The S. cerevisiae respiratory SC is composed of complexes III2 (CIII, dimer of cytochrome bc1) and IV (CIV, Cyt c oxidase) with CIII flanked on each side by CIV in the core tetrameric SC (IV1III2IV1). CL is distinguished from other phospholipids by its unique dimeric structure containing two phosphates, four fatty acids and a free hydroxyl at the 2-position of the glycerol linking the two phosphatidyl groups. This unique dimeric structure makes CL ideal for supporting the organization of individual protein subunits into multi-subunit complexes, as well as individual complexes into supercomplex (SC) molecular machines, such as the mitochondrial respirasome. A presumed advantage in SC formation is bringing active sites of CIII and CIV in close proximity to each other to facilitate Cyt c shuttling of electrons. Here we show that anionic phospholipids interact with positive amino acids and appear to nucleate a phospholipid domain at the interface between the individual complexes, which dampen charge repulsion and further stabilize interaction, respectively, between individual complexes.

To address whether PG substitutes for CL in SC formation, we performed single-particle cryo-EM analysis of the trimeric SC purified from CRD1∆ cells. There was no density in the region of the CRD1∆ density map corresponding to the position of the Qcr10 subunit of CIII in the WT SC density map; we assume that this subunit was lost during purification. Densities for UQ6 were found only at Qi sites. The Qo sites were empty, which may be due to use of chromatography for purification resulting in the oxidation of UQ6. Analysis of the cryo-EM density for Rip1 subunit of CIII showed that both the hinge region and the head domain displayed weaker or less ordered density when compared to the WT. Our structural determination of the trimeric SC from CRD1∆ cells shows the presence of the anionic phospholipid PG at all CL positions found in the WT SC, which has been postulated but never demonstrated. PGT501J/j appears to replace the internal CLs in each monomer of CIII surprisingly resulting in little noticeable structural changes for CIII. PGT601K appears to only interact with CIV unlike CDL601K which interacts with both CIII and CIV. However, there is no interaction with Lys51 of Rip1 since PGT lacks a second phosphate. However, there were significant differences as to which amino acids interact with PG and none of the PGs formed interactions that bridge CIII and CIV.

>[2x]MLRTVTSKTVSNQFKRSLATAVATPKAEVTQLSNGIVVATEHNPSAHTASVGVVFGSGAANENPYNNGVSNLWKNIFLSKENSAVAAKEGLALSSNISRDFQSYIVSSLPGSTDKSLDFLNQSFIQQKANLLSSSNFEATKKSVLKQVQDFEENDHPNRVLEHLHSTAFQNTPLSLPTRGTLESLENLVVADLESFANNHFLNSNAVVVGTGNIKHEDLVNSIESKNLSLQTGTKPVLKKKAAFLGSEVRLRDDTLPKAWISLAVEGEPVNSPNYFVAKLAAQIFGSYNAFEPASRLQGIKLLDNIQEYQLCDNFNHFSLSYKDSGLWGFSTATRNVTMIDDLIHFTLKQWNRLTISVTDTEVERAKSLLKLQLGQLYESGNPVNDANLLGAEVLIKGSKLSLGEAFKKIDAITVKDVKAWAGKRLWDQDIAIAGTGQIEGLLDYMRIRSDMSMMRW;>[2x]MLSAARLQFAQGSVRRLTVSARDAPTKISTLAVKVHGGSRYATKDGVAHLLNRFNFQNTNTRSALKLVRESELLGGTFKSTLDREYITLKATFLKDDLPYYVNALADVLYKTAFKPHELTESVLPAARYDYAVAEQCPVKSAEDQLYAITFRKGLGNPLLYDGVERVSLQDIKDFADKVYTKENLEVSGENVVEADLKRFVDESLLSTLPAGKSLVSKSEPKFFLGEENRVRFIGDSVAAIGIPVNKASLAQYEVLANYLTSALSELSGLISSAKLDKFTDGGLFTLFVRDQDSAVVSSNIKKIVADLKKGKDLSPAINYTKLKNAVQNESVSSPIELNFDAVKDFKLGKFNYVAVGDVSNLPYLDEL;>MLGIRSSVKTCFKPMSLTSKRLISQSLLASKSTYRTPNFDDVLKENNDADKGRSYAYFMVGAMGLLSSAGAKSTVETFISSMTATADVLAMAKVEVNLAAIPLGKNVVVKWQGKPVFIRHRTPHEIQEANSVDMSALKDPQTDADRVKDPQWLIMLGICTHLGCVPIGEAGDFGGWFCPCHGSHYDISGRIRKGPAPLNLEIPAYEFDGDKVIVG[2x];>MSFSSLYKTFFKRNAVFVGTIFAGAFVFQTVFDTAITSWYENHNKGKLWKDVKARIAAGDGDDDDE[2x];>MPQSFTSIARIGDYILKSPVLSKLCVPVANQFINLAGYKKLGLKFDDLIAEENPIMQTALRRLPEDESYARAYRIIRAHQTELTHHLLPRNEWIKAQEDVPYLLPYILEAEAAAKEKDELDNIEVSK[2x];>[2x]MGMLELVGEYWEQLKITVVPVVAAAEDDDNEQHEEKAAEGEEKEEENGDEDEDEDEDEDDDDDDDEDEEEEEEVTDQLEDLREHFKNTEEGKALVHHYEECAERVKIQQQQPGYADLEHKEDCVEEFFHLQHYLDTATAPRLFDKLK;>MGPPSGKTYMGWWGHMGGPKQKGITSYAVSPYAQKPLQGIFHNAVFNSFRRFKSQFLYVLIPAGIYWYWWKNGNEYNEFLYSKAGREELERVNV[2x];>[2x]MAFRKSNVYLSLVNSYIIDSPQPSSINYWWNMGSLLGLCLVIQIVTGIFMAMHYSSNIELAFSSVEHIMRDVHNGYILRYLHANGASFFFMVMFMHMAKGLYYGSYRSPRVTLWNVGVIIFILTIATAFLGYCCVYGQMSHWGATVITNLFSAIPFVGNDIVSWLWGGFSVSNPTIQRFFALHYLVPFIIAAMVIMHLMALHIHGSSNPLGITGNLDRIPMHSYFIFKDLVTVFLFMLILALFVFYSPNTLGHPDNYIPGNPLVTPASIVPEWYLLPFYAILRSIPDKLLGVITMFAAILVLLVLPFTDRSVVRGNTFKVLSKFFFFIFVFNFVLLGQIGACHVEVPYVLMGQIATFIYFAYFLIIVPVISTIENVLFYIGRVNK;> MVQRWLYSTNAKDIAVLYFMLAIFSGMAGTAMSLIIRLELAAPGSQYLHGNSQLFNVLVVGHAVLMIFFLVMPALIGGFGNYLLPLMIGATDTAFPRINNIAFWVLPMGLVCLVTSTLVESGAGTGWTVYPPLSSIQAHSGPSVDLAIFALHLTSISSLLGAINFIVTTLNMRTNGMTMHKLPLFVWSIFITAFLLLLSLPVLSAGITMLLLDRNFNTSFFEVSGGGDPILYEHLFWFFGHPEVYILIIPGFGIISHVVSTYSKKPVFGEISMVYAMASIGLLGFLVWSHHMYIVGLDADTRAYFTSATMIIAIPTGIKIFSWLATIHGGSIRLATPMLYAIAFLFLFTMGGLTGVALANASLDVAFHDTYYVVGHFHYVLSMGAIFSLFAGYYYWSPQILGLNYNEKLAQIQFWLIFIGANVIFFPMHFLGINGMPRRIPDYPDAFAGWNYVASIGSFIATLSLFLFIYILYDQLVNGLNNKVNNKSVIYNKAPDFVESNTIFNLNTVKSSSIEFLLTSPPAVHSFNTPAVQS;>[2x]MFSNLSKRWAQRTLSKSFYSTATGAASKSGKLTQKLVTAGVAAAGITASTLLYADSLTAEAMTAAEHGLHAPAYAWSHNGPFETFDHASIRRGYQVYREVCAACHSLDRVAWRTLVGVSHTNEEVRNMAEEFEYDDEPDEQGNPKKRPGKLSDYIPGPYPNEQAARAANQGALPPDLSLIVKARHGGCDYIFSLLTGYPDEPPAGVALPPGSNYNPYFPGGSIAMARVLFDDMVEYEDGTPATTSQMAKDVTTFLNWCAEPEHDERKRLGLKTVIILSSLYLLSIWVKKFKWAGIKTRKFVFNPPKPRK;> MLCQQMIRTTAKRSSNIMTRPIIMKRSVHFKDGVYENIPFKVKGRKTPYALSHFGFFAIGFAVPFVACYVQLKKSGAF;> MANKVIQLQKIFQSSTKPLWWRHPRSALYLYPFYAIFAVAVVTPLLYIPNAIRGIKAKKA;> MTHLERSRHQQHPFHMVMPSPWPIVVSFALLSLALSTALTMHGYIGNMNMVYLALFVLLTSSILWFRDIVAEATYLGDHTMAVRKGINLGFLMFVLSEVLIFAGLFWAYFHSAMSPDVTLGACWPPVGIEAVQPTELPLLNTIILLSSGATVTYSHHALIAGNRNKALSGLLITFWLIVIFVTCQYIEYTNAAFTISDGVYGSVFYAGTGLHFLHMVMLAAMLGVNYWRMRNYHLTAGHHVGYETTIIYTHVLDVIWLFLYVVFYWWGV;> MLDLLRLQLTTFIMNDVPTPYACYFQDSATPNQEGILELHDNIMFYLLVILGLVSWMLYTIVMTYSKNPIAYKYIKHGQTIEVIWTIFPAVILLIIAFPSFILLYLCDEVISPAMTIKAIGYQWYWKYEYSDFINDSGETVEFESYVIPDELLEEGQLRLLDTDTSMVVPVDTHIRFVVTAADVIHDFAIPSLGIKVDATPGRLNQVSALIQREGVFYGACSELCGTGHANMPIKIEAVSLPKFLEWLNEQ;> MLSRAIFRNPVINRTLLRARPGAYHATRLTKNTFIQSRKYSDAHDEETFEEFTARYEKEFDEAYDLFEVQRVLNNCFSYDLVPAPAVIEKALRAARRVNDLPTAIRVFEALKYKVENEDQYKAYLDELKDVRQELGVPLKEELFPSSS;> MTIAPITGTIKRRVIMDIVLGFSLGGVMASYWWWGFHMDKINKREKFYAELAERKKQEN;> MFRQCAKRYASSLPPNALKPAFGPPDKVAAQKFKESLMATEKHAKDTSNMWVKISVWVALPAIALTAVNTYFVEKEHAEHREHLKHVPDSEWPRDYEFMNIRSKPFFWGDGDKTLFWNPVVNRHIEHDD;> MLSLRQSIRFFKPATRTLCSSRYLLQQKPVVKTAQNLAEVNGPETLIGPGAKEGTVPTDLDQETGLARLELLGKLEGIDVFDTKPLDSSRKGTMKDPIIIESYDDYRYVGCTGSPAGSHTIMWLKPTVNEVARCWECGSVYKLNPVGVPNDDHHH;> MADQENSPLHTVGFDARFPQQNQTKHCWQSYVDYHKCVNMKGEDFAPCKVFWKTYNALCPLDWIEKWDDQREKGIFAGDINSD;> MFFSQVLRSSARAAPIKRYTGGRIGESWVITEGRRLIPEIFQWSAVLSVCLGWPGAVYFFSKARKA;> MLRNTFTRAGGLSRITSVRFAQTHALSNAAVMDLQSRWENMPSTEQQDIVSKLSERQKLPWAQLTEPEKQAVWYISYGEWGPRRPVLNKGDSSFIAKGVAAGLLFSVGLFAVVRMAGGQDAKTMNKEWQLKSDEYLKSKNANPWGGYSQVQSK>LDYLTGILITRHSQSETVPACSAGHTELWTGYSLLYVDGNDYAHNQDLGSPGSCVPRFSTLPVLSCGQNNVCNYASRNDKTFWLTTNAAIPMMPVENIEIRQYISRCVVCEAPANVIAVHSQTIEVPDCPNGWEGLWIGYSFLMHTAVGNGGGGQALQSPGSCLEDFRATPFIECNGAKGTCHFYETMTSFWMYNLESSQPFERPQQQTIKAGERQSHVSRCQVCMKNSS[4x];>APKSRGFIFARHSQSVHVPQCPANTNLLWEGYSLSGNVAASRAVGQDLGQSGSCMMRFTTMPYMLCDITNVCHFAQNNDDSLWLSTAEPMPMTMTPIQGRDLMKYISRCVVCETTTRIIALHSQSMSIPDCPGGWEEMWTGYSYFMSTLDNVGGVGQNLVSPGSCLEEFRAQPVIECHGHGRCNYYDALASFWLTVIEEQDQFVQPRQQTLKADFTSKISRCTVCRRRGN[2x]

Collagen IV is an essential structural protein in all metazoans. It provides a scaffold for the assembly of basement membranes, a specialized form of extracellular matrix, which anchors and signals cells and provides microscale tensile strength. Scaffolds are composed of α-chains that coassemble into triple-helical protomers of distinct chain compositions, which in turn oligomerize into supramolecular scaffolds. We solved the crystal structure of the NC1 hexamer, determined the chain composition of protomers, and found that Drosophila adapted an evolutionarily unique mechanism of scaffold assembly that requires divalent cations.

We used Drosophila pellet to extract and purify endogenous NC1 hexamer as described in Experimental procedures. Collectively, Drosophila collagen IV does form the hexamer, which contains both Cg25c and Vkg chains; and the Vkg “tail” sequence (not found in mammals) is not an integral part of the NC1 hexamer. Isolation of endogenous NC1 hexamer from Drosophila pellet showed the presence of both Cg25c and Vkg chains. We were able to obtain diffracting crystals of tissue-extracted NC1 hexamer (at 2.98 Å resolution) and CVC trimer (at 1.75 Å resolution) and solved their atomic structures. We solved the crystal structures of tissue-extracted and recombinant NC1 hexamers and found that the tissue-extracted complex is indeed a heterotrimer of the same composition as the recombinant CVC single-chain construct. RMSD of superimposed recombinant and tissue-extracted structures of Drosophila NC1 hexamer is 0.43 Å between 1346 pruned atom pairs (across all 1351 pairs: 0.47 Å). A slight difference between CVC hexamer and tissue-extracted hexamer might be due to extra linkers and FLAG-tag sequences in CVC and sulfilimine cross-links in tissue-extracted hexamer. Out of 12 chloride ions found at the hexamer interface in mammals only four were found in Drosophila. Only Cg25c chains were found to contain chloride ions, while Vkg chains contain water molecules instead. In the solved crystal structures, we indeed observed four pairs of double salt bridges from R76(1626) of each Cg25c to either E173(1723) of Cg25c or E175(1685) of Vkg.>[2x]GLVPRGSHMMDTRPIGFLDSGVGGLTVVCELIRQLPHEKIVYIGDSARAPYGPRPKKQIKEYTWELVNFLLTQNVKMIVFACNTATAVAWEEVKAALDIPVLGVVLPGASAAIKSTTKGQVGVIGTPMTVASDIYRKKIQLLAPSIQ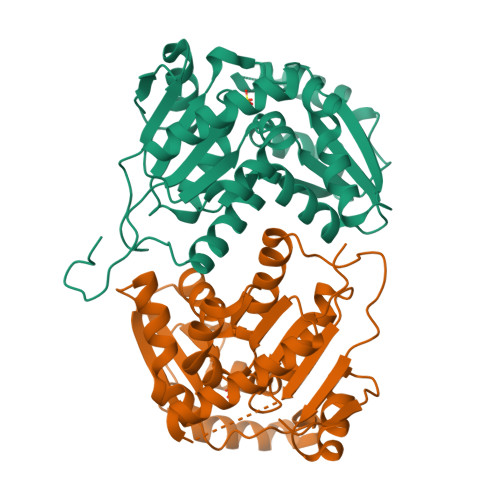VRSLACPKFVPIVESNEMCSSIAKKIVYDSLAPLVGKIDTLVLGCTHYPLLRPIIQNVMGPSVKLIDSGAECVRDISVLLNYFDINGNYHQKAVEHRFFTTANPEIFQEIASIWLKQKINVEHVTL> AFTFRYSPSLYTWFL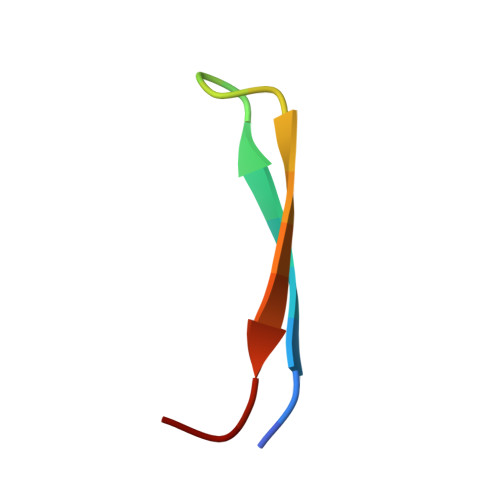FPCG>[6x]MSLQKRVALVTGGSGGLGRVHALTLAQNGADVAVTGNRNIDKAESVANEIRALGRKALAIKVDVSNEDEVNEGVEKIKKELGSVDILVNNAASGIVRATLIEKTAKEDWDQDLRVNLTGAFNCIKAVIPDMKKNNWGRIINISSVTGTMGGSGQCSYATTKAGLIGLTKTVALEGARYNITCNALVLGVFGGRGREDSSFYDVAEPFRERIIKRTAMRRPGDPKELSNVLAFLASDEASYVTGDAIV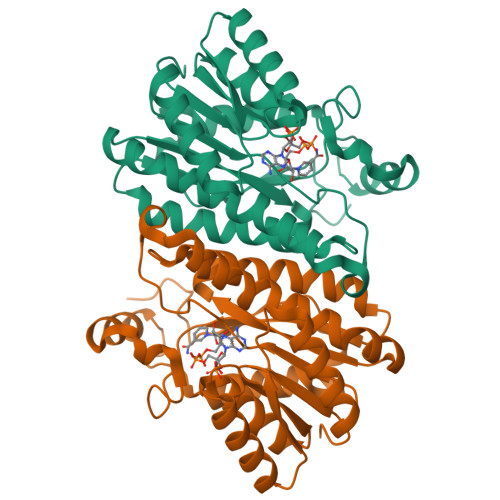VGGGIDLFTF> 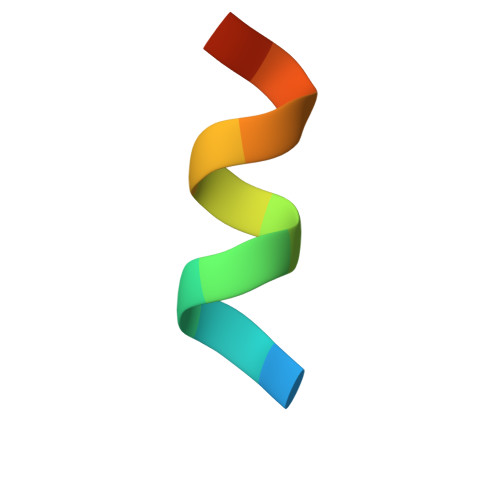KHKILHRLLQASS>[2x]MIPHSWICEKHILWLKDYKNSSNWKLFKECWKQGQPAVVSGVHKKMNISLWKAESISLDFGDHQADLLNCKDSIISNANVKEFWDGFEEVSKRQKNKSGETVVLKLKDWPSGEDFKTMMPARYEDLLKSLPLPEYCNPEGKFNLASHLPGFFVRPDLGPRLCSAYGVVAAKDHDIGTTNLHIEVSDVVNILVYVGIAKGNGILSKAGILKKFEEEDLDDILRKRLKDSS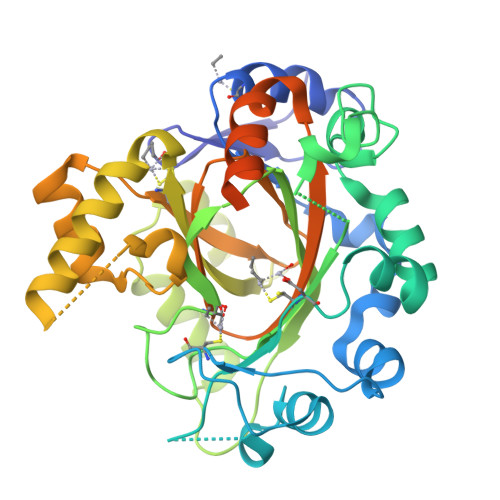EIPGALWHIYAGKDVDKIREFLQKISKEQGLEVLPEHDPIRDQSWYVNKKLRQRLLEEYGVRTCTLIQFLGDAIVLPAGALHQVQNFHSCIQVTEDFVSPEHLVESFHLTQELRLLKEEINYDDKLQVKNILYHAVKEMVRALKIHEDEVEDMEENAENLYFQ> GAMGISLPLLKQDDWLSSSKPFGSSTPNV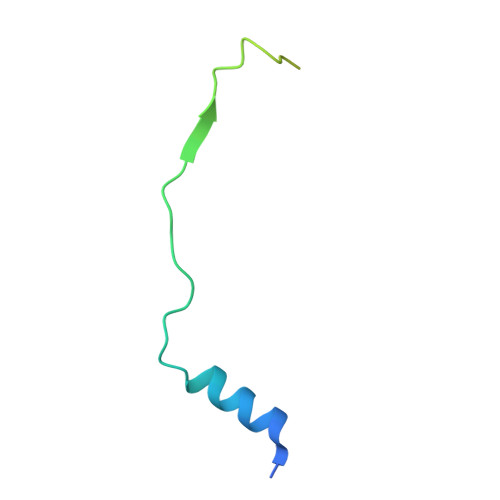VIEFDSDDDGDDFSNSKIEQSNLEKPPSNSENGGSHHHHHH> MTSRKKVLLKVIILGDSGVGKTSLMNQYVNKKFSNQYKATIGADFLTKEVMVDDRLVTMQIWDTAGQERFQSLG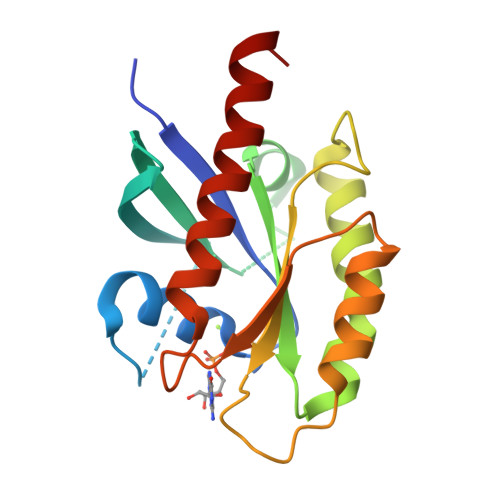VAFYRGADCCVLVFDVTAPNTFKTLDSWRDEFLIQASPRDPENFPFVVLGNKIDLENRQVATKRAQAWCYSKNNIPYFETSAKEAINVEQAFQTIARNALKQETEVELYNE> MSKRYFVTGTDTEVGKTVASCALLQAAKAAGYRTAGYKPVASGSEKTPEGLRNSDALALQRNSSLQLDYATVNPYTFAEPTSPHIISAQEGRPIESLVMSAGLRALEQQADWVLVEGAGGWFTPLSDTFTFADWVTQEQLPVILVVGVKLGCINHAMLTAQVIQHAGLTLAGWVA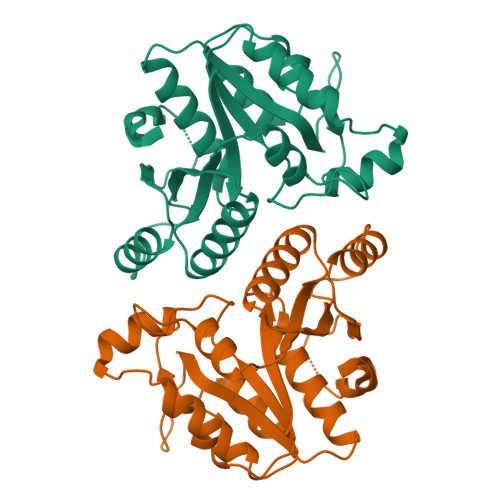NDVTPPGKRHAEYMTTLTRMIPAPLLGEIPWLAEAATGKYINLALL3-[4-[[1-[(4-chloranyl-1H-indol-2-yl)methyl]-3,7-dimethyl-2,6-bis(oxidanylidene)purin-8-yl]amino]-6-methyl-pyrimidin-2-yl]propanoic 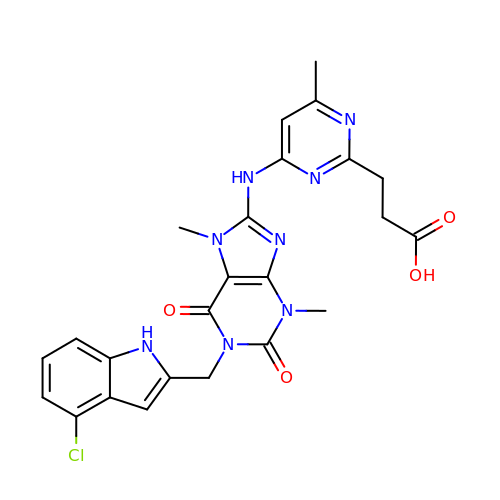acid | C24 H23 Cl N8 O4 | ILEKCBRCJDWEIR-UHFFFAOYSA-N>[2x]MSSRVPILKVDDYWVVAIEETLHDQSVIQFKEELLHNITGVAGKGLVIDISALEVVDSFVTRVLIEISRLAELL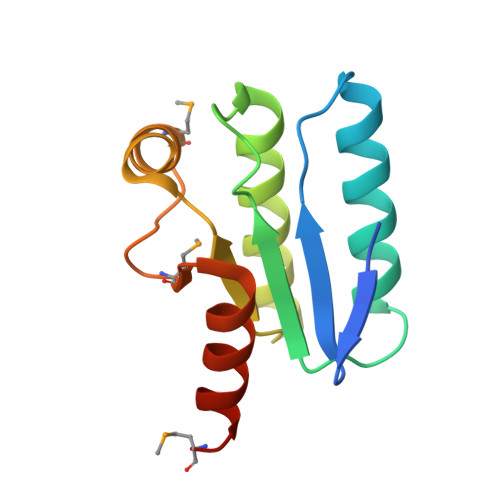GLPFVLTGIKPAVAITLTEMGLDLRGMATALNLQKGLDKLKNLARMEQR> SQAESKEWYHASLTRAQAEHMLMRVPRDGAFLVRKRNEPNSYAISFRAEGKIKHCRVQQEGQTVMLGNSEFDSLV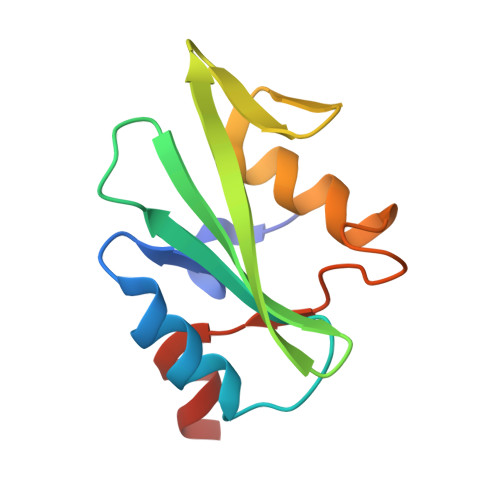DLISYYEKHPLYRKMKLRYPINEEALEKIGT> SMSLNIITVTLNMEKYNFLGI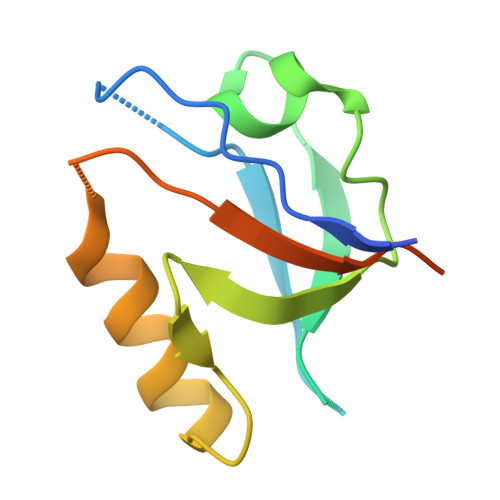SIVGQSNERGDGGIYIGSIMKGGAVAADGRIEPGDMLLQVNDMNFENMSNDDAVRVLRDIVHKPGPIVLTVAKSGGGGSTFSLWQDIP>MRGSHHHHHHGSMAEGEEYDKILVLNFGSQYFHLIVKRLNNIKIFSETKDYGVELKDIKDMNIKGVILSGGPYSVTEAGSPHLKKEVFEYFLEKKIPIFGICYGMQEIAVQMNGEVKKSKTSEYGCTDVNILRNDNINNITYCRNFGDSSSAMDLYSNYKLMNETCCLFENIKSDITTVWMNHNDEVTKIPENFYLVSSSENCLICSIYNKEYNIYGVQYHPEVYESLDGELMFYNFAYNICKCKKQFDPIRYHELELKNIEKYKHDHYVIAAMSGGIDSTVAAAYTHKIFKERFFGIFIDNGLLRKNEAENVYTFLKSTFPDMNITKIDASENFLSNLQGVTDPEQKRKIIGKLFIEEFEKAVNNIDIDINKTFLLQGTLYPDIIESKCSKNLSDTIKTHHNVGGLPKNLKFKLFEPFKYLFKDDVKTLSRELNLPEEITNRHPFPGPGLAIRVIGEINKHKLNILREVDDIFINDLKQYGLYNQISQAFAVLLSSKSVGVRGDARSYDYVCVLRAVKTSSFMTANWYQIPYDILDKITTRILSEVKGVNRILYDVSSKPPATIEFE[2x]

GMP synthesis proceeds through two steps, the first being the conversion of IMP to xanthine monophosphate (XMP) catalysed by IMP dehydrogenase followed by GMPS (guanosine 5′-monophosphate synthetase; EC 6.3.5.2) converting XMP to GMP4. GMPS is a class-I (trpG-type) amidotransferase in which the catalytic reaction occurs in two physically distant domains, a GATase (glutamine amidotransferase) domain and an ATPPase (ATP pyrophosphatase) domain5. Hydrolysis of glutamine to glutamate and ammonia occurs in the GATase domain, whereas formation of the intermediate AMP-XMP from ATP and XMP occurs in the ATPPase domain. Ammonia generated in the GATase domain attacks the intermediate to generate GMP.

We purified and crystallized PfGMPS, PfGMPS_C89A and PfGATase, and solved their structures by molecular replacement to resolutions of 3.6, 3.15 and 2.6 Å, respectively. The 108 C-terminal residues of the ATPPase domain are involved in dimerization. Interestingly, the nucleotide-binding site of PfGMPS comprises residues from two adjacent monomers, strongly suggesting that the dimer is essential for enzymatic activity. Small angle X-ray scattering (SAXS) confirmed the dimeric structure of PfGMPS in solution corresponding to the active form of the enzyme, as seen from the good fit of the dimer crystal structure superimposed onto the calculated 17 Å resolution PfGMPS SAXS envelope. Upon superposition of the PfGMPS- (conformational state I) and PfGMPS_C89A/Gln (conformational state II) dimer structures, the two ATPPase domains remain invariant, whereas the two GATase domains differ by an 85° rotation and a 3 Å translation when going from states I to II. Probably binding of ATP and XMP by changing the conformation of helix 371–375 could be responsible for the interface rearrangement. It also seems plausible that the charge-mediated interaction between Glu374 and His20, along with the hydrophobic interface contributes to stabilize PfGMPS in the conformation observed for ligand-free and XMP-bound enzymes. His20 (in close vicinity of Glu374 in the apo PfGMPS structure) was mutated to Ala, giving a 23% drop in leaky activity. As the structure of PfGMPS shows inter-domain interaction via Glu374 and His20, the rate of adenyl-XMP formation in PfGMPS_H20A upon mixing the enzyme with ATP and XMP was measured. A progress curve with a single slope and an apparent rate constant of 96±6 min−1 was obtained, and the 1.6-fold drop of the rate constant validates the inter-domain interaction seen in the structure.Tick-borne encephalitis virus (Orthoflavivirus encephalitidis, TBEV) is an enveloped single-stranded (+)RNA virus belonging to the Orthoflavivirus genus. Orthoflavivirus particles have icosahedral symmetry with a diameter of about 50 nm and a genome of about 11 kb. The glycoprotein shell of the mature infectious virion consists of 180 copies of each of membrane-anchored E (496 amino acid residues) and M proteins (75 amino acid residues). Envelope proteins E orchestrate the early stages of viral infection, virus entry into the cell and receptor-mediated endocytosis.

Here we report the refined single-particle cryo-electron microscopy (cryo-EM) structure of the inactivated mature TBEV vaccine strain Sofjin–Chumakov (Far-Eastern subtype) at a resolution of 3.0 Å. A clear electron density was observed for the E protein ectodomain shell showing the arrangement of antiparallel dimers on the surface of the virion into the common “herringbone” pattern with icosahedral symmetry (residues 1–396). Residues 14–18 (domain I) were not resolved in two of three independent subunits. We also did not observe electron density for any parts of the M protein as well as for stem and anchor regions of E protein, in contrast to the previously published TBEV structures. The absence of electron density below the E protein ectodomain shell in our structure of inactivated TBEV suggests that formaldehyde linking likely causes rigidification of the ectodomains, which start to act as a sort of “hull,” while membrane-associated domains become less ordered. Thus two types of dimers are present: symmetric dimer formed by twofold icosahedral axis-related subunits, and asymmetric dimer formed by E3 and E5 subunits. We calculated the volume and surface area for these cavities for E5–E3 dimers in all the three TBEV structures, as well as for Zika virus and Japanese encephalitis virus. iTBEV had the smallest surface area and volume for both cavities compared to those in TBEV-Kuutsalo and TBEV-Hypr, consistent with the largest buried surface area between the subunits. Thus one may suggest that all the major structural epitopes should be conserved in the vaccine particles and not destroyed by the formaldehyde inactivation. Our structure directly confirms this hypothesis: for all the previously described complexes of TBEV envelope proteins with antibodies, resolved by different methods (X-ray crystallography or cryo-EM), the epitope structure is reproduced by our data, meaning that formaldehyde inactivation is soft enough and suitable for the virus structure studies in general. While intact TBEV conformationally rearranges at pH 6.0 and decreases its ability to bind mAbs, inactivated TBEV binds them with the same efficiency at pH 6.0 and 7.8, suggesting that its conformation is not dependent on the pH due to formaldehyde-induced cross-linking of the envelope proteins.

>[3x]SRCTHLENRDFVTGTQGTTRVTLVLELGGCVTITAEGKPSMDVWLDSIYQENPAKTREYCLHAKLSDTKVAARCPTMGPATLAEEHQSGTVCKRDQSDRGWGNHCGLFGKGSIVTCVKASCEAKKKATGHVYDANKIVYTVKVEPHTGDYVAANETHSGRKTASFTVSSEKTILTMGDYGDVSLLCRVASGVDLAQTVILELDKTSEHLPTAWQVHRDWFNDLALPWKHEGAQNWNNAERLVEFGAPHAVKMDVYNLGDHTGVLLKSLAGVPVAHIDGTKYHLKSGHVTCEVGLEKLKMKGLTYTMCDKTKFTWKRIPTDSGHDTVVMEVAFSGTKPCRIPVRAVAHGSPDVNVAMLITPNPIIENNGGGFIEMQLPPGDNIIYVGELSHQWFQKG6-amino-3,7-dihydro-2H-purin-2-one 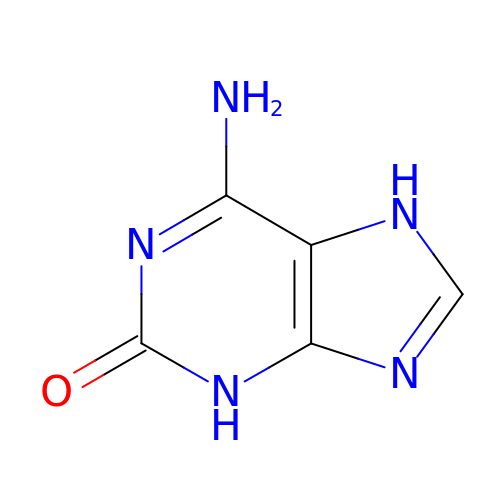| C5 H5 N5 O | DRAVOWXCEBXPTN-UHFFFAOYSA-N>MAFPIPARQLFIDGEWREPIKKNRIPVINPSTEEIIGDIPAATAEDVEVAVVAARRAFRRNNWSATSGAHRATYLRAIAAKITEKKDHFVKLETIDSGKPFDEAVLDIDDVASCFEYFAGQAEALDGKQKAPVTLPMERFKSHVLRQPLGVVGLISPWNYPLLMATWKIAPALAAGCTAVLKPSELASVTCLEFGEVCNEVGLPPGVLNILTGLGPDAGAPLVSHPDVDKIAFTGSSATGSKVMASAAQLVKPVTLELGGKSPIVVFEDVDIDKVVEWTIFGCFWTNGQIASATSRLLVHESIAAEFVDKLVKWTKNIKISDPFEEGCRLGPVISKGQYDKIMKFI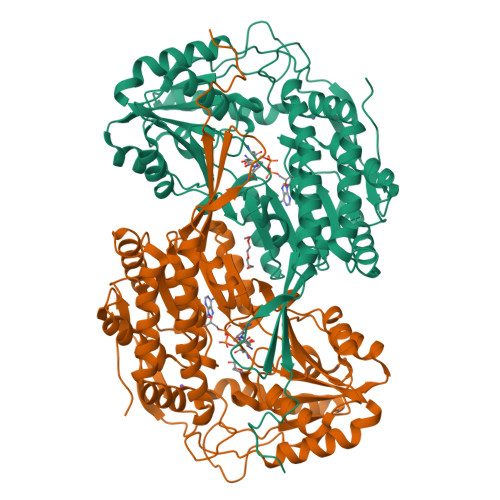STAKSEGATILYGGSRPEHLKKGYYIEPTIVTDISTSMQIWKEEVFGPVLCVKTFSSEDEAIALANDTEYGLAAAVFSNDLERCERITKALEVGAVWVNCSQPCFVQAPWGGIKRSGFGRELGEWGIQNYLNIKQVTQDISDEPWGWYKSP[4x]>APASLLPPAPEHSPPSSPLTQPPEGPKFPRVKNWEVGSITYDTLSAQAQQDGPCTPRRCLGSLVFPRKLQGRPSPGPPAPEQLLSQARDFINQYYSSIKRSGSQAHEQRLQEVEAEVAATGTYQLRESELVFGAKQAWRNAPRCVGRIQWGKLQVFDARDCRSAQEMFTYICNHIKYATNRGNLRSAITVFPQRCPGRGDFRIWNSQLVRYAGYRQQDGSVRGDPANVEITELCIQHGWTPGNGRFDVLPLLLQAPDEPPELFLLPPELVLEVPLEHPTLEWFAALGLRWYALPAVSNMLLEIGGLEFPAAPFSGWYMSTEIGTRNLCDPHRYNILE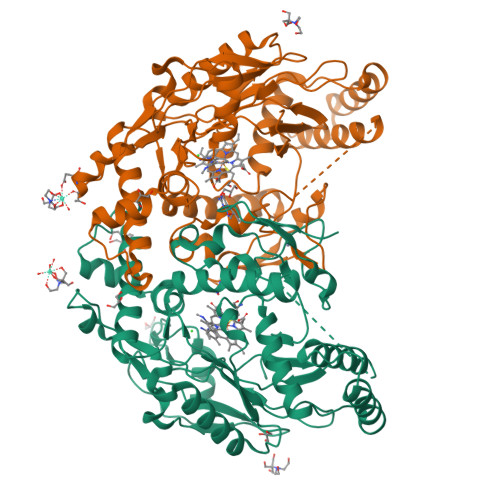DVAVCMDLDTRTTSSLWKDKAAVEINVAVLHSYQLAKVTIVDHHAATASFMKHLENEQKARGGCPADWAWIVPPISGSLTPVFHQEMVNYFLSPAFRYQPDPW[4x]> MTQTITVIRGDGIGPEIMDATLFVLDALQAGLTYEYADAGLVALEKHGDLLPESTLASITKNKVALKSPLTTPVGEGFSS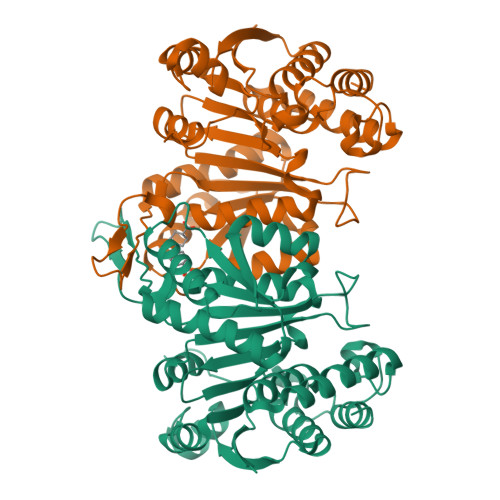INVAMRRKFDLYANVRPAKSFPNTKSRFADGVDLITVRENTEGAYLSEGQEVSADGEVAVSGARVTRKGSERIVRYAFDLARATGRKKVTAVHKANIIKSTSGLFLKVARDVATQYPEIEFQEMIVDNTCMQLVMRPEQFDIIVTTNLFGDIISDLCAGLVGGLGLAPGANIGVDAAIFEAVHGSAPDIAGQGKANPCALLLGAAQMLDHIGQPQNAERLREAIVATLEAKDSLTPDLGGTGNTMGFAKAIASRL>MDFSRNLYDIGEQLDSEDLASLKFLSLDYIPQRKQEPIKDALMLFQRLQEKRMLEESNLSFLKELLFRINRLDLLITYLNTRKEEMERELQTPGRAQISAYRVMLYQISEEVSRSELRSFKGGLQEEISKCKLDDDMNLLDIFIEMEKRVILGEGKLDILKRVCAQINKSLLKIINDYEEFSKER[5x];>MSAEVIGQVEEALDTDEKEMLLFLCRDVAIDVVPPNVRDLLDILRERGKLSVGDLAELLYRVRRFDLLKRILKMDRKAVETHLLRNPHLVSDYRVLMAEIGEDLDKSDVSSLIFLMKDYMGRGKISKEKSFLDLVVELEKLNLVAPDQLDLLEKCLKNIHRIDLKTKIQKYKQSVQGAGTS[4x];> MDPFLVLLGSVSSSLSSSELTELKFLCLGRVGKRKLERVQSGLDLFSMLLEQNDLEPGHTELLRELLASLRRHDLLRRVDDFEAGAAAGAAPGEEDLCAAFNVICDNVGKDWRRLARQLKVSDTKIDSIEDRYPRNLTERVRESLRIWKNTEKENATVAHLVGALRSCQMNLVADLVQEVQQARDLQNRSGAMSPMSWNSDASTSEASLEHHHHHH

Fas-associated protein with death domain (FADD), procaspase-8, and cellular FLICE-inhibitory proteins (cFLIP) assemble through death-effector domains (DEDs), directing death receptor signaling towards cell survival or apoptosis. In this work, we present the crystal and cryo-EM structures of ternary FADD-Casp-8-cFLIP DED complexes, unveiling FADD-FADD, FADD-Casp-8, FADD-cFLIP, Casp-8-cFLIP, and cFLIP-cFLIP DED assemblies in a complex. The atomic coordinates depict how FADDDED and Casp-8tDED could assemble a helical 1:5 and 3:3 intermediate complexes, and how these FADD-Casp-8 intermediate complexes are targeted and capped by four cFLIPtDED molecules. The resultant helical Casp-8tDED-cFLIPtDED hetero-double layer appears to locally activate Casp-8.

We successfully reconstituted the ternary complex FADDFuL_H9G-Casp-8tDED_F122G/L123G-cFLIPtDED_H7G complex, henceforth referred to as the FAFuL_H9G-C8FGLG-CFH7G complex. Subsequently, we obtained the protein crystals and determined the crystal structure at 3.1 Å resolution using the MR-SAD method, in which FADD DD is not visible. Notably, the crystal structure reveals a 1:5:4 stoichiometry for the FAFuL_H9G-C8FGLG-CFH7G complex. The single-FADD complex structure unveils additional FADDDED-Casp-8tDED assembly, in which Casp-8tDED assembles a type III-II-III CSS-mediated pentamer, containing Casp-8tDED molecules C8a, C8b, C8c, C8d, and C8e. In the 1:5:4 FAFuL_H9G-C8FGLG-CFH7G complex structure, three Casp-8tDED molecules C8c, C8d, and C8a provide, respectively, a type Ia, a type IIa, and a type IIIa surfaces, while FADDDED molecule FAl provides a type IIa and a type IIIa surfaces to complete the CBS to recruit cFLIPtDED_H7G molecule CFk. In the single-FADD structure, the halt of Casp-8 filamentation at the upper end results from the inability of the CSS of Casp-8tDED molecule C8e to bind and stabilize another Casp-8 tDED when there’s no FADD in the adjoining space.>[7x]MSNETIVIDIKGAVQHPGVYEMRTGDRVSQAIEKAGGTSEQADEAQVNLAEILQDGTVVYIPKKGEETAVQQGGGGSVQSDGGKGALVNINTATLEELQGISGVGPSKAEAIIAYREENGRFQTIEDITKVSGIGEKSFEKIKSSITVKLEHHHHHH

ComEA, a DNA-binding protein widely conserved in transformable bacteria, is required for this uptake step. Following this contact with the tpilus, the movement of tDNA into the periplasm is driven by its interaction with the widely conserved periplasmic protein ComEA. A ComEABs contains an N-terminal transmembrane region, a previously unidentified OD, and a C-terminal DNA-binding domain. We show that this domain drives ComEA oligomerization, and that oligomerization is required for genetic transformation.

To gain mechanistic insight into the function of ComEA, we cloned, overexpressed, purified, and determined the X-ray crystal structures of ComEABs and ComEAGs to 3.20 Å and 3.05 Å resolution, respectively. No electron density was evident for the ComEABs DNA-binding domain or linker region, but there was clear density corresponding to a previously undescribed domain (amino acids 60–122). There are seven of these domains arranged head-to-tail in the ComEABs crystallographic asymmetric unit, and we named this region the oligomerization domain (OD). More specifically, in the ComEABs structure, the seven-membered asymmetric unit uses the OD multimerization interface to form a 14-membered head-to-tail ring around the crystallographic two-fold axis. We measured this in vivo by comparing B. subtilis transformation in strains containing wild-type ComEABs; ComEABs-D111N, which disrupts a conserved intermolecular salt-bridge between D111 and R83 (corresponding to ComEAGs Asp113 and Arg85); ComEABs-A106Y (corresponding to ComEAGs-A108Y), which sterically blocks OD multimerization; and ComEA-ΔOD, containing a deletion of the entire OD, while leaving intact both the transmembrane region and the DNA-binding domain. In comparison to wild-type ComEABs, ComEABs-D111N reduced B. subtilis transformation nearly 100-fold. Even more striking were the ComEABs-A106Y and ComEA-ΔOD mutations that reduced B. subtilis transformation about 1,000-fold, a phenotype equivalent to that of a complete comEA deletion. As shown in, the A106Y mutation prevents stable DNA association with competence-expressing cells, which we have shown previously required uptake to the periplasm. To begin to understand the importance of ComEA sidechain interactions to DNA binding and ComEA function, we mutated some of the corresponding interfacial residues in ComEABs (e.g., ComEABs K164 and K193) to alanine and tested their effect on transformation in B. subtilis. Western blot analysis showed that wild-type ComEABs and the ComEABs proteins containing mutations in the HhH motifs were expressed to similar levels. These in vivo studies also showed that the K164A and K199A mutations caused more than a 2-log decrease in transformation, in contrast to the reproducible 2-4-fold effects of K193A and K197A.> GLPVLNTPGSNQ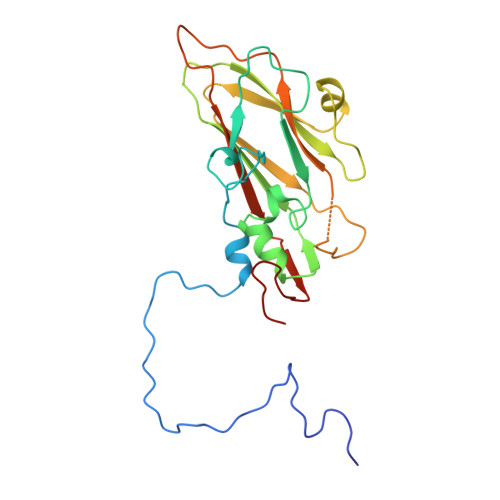YLTADNYQSPCAIPEFDVTPPIDIPGEVRNMMELAEIDTMIPLNLTNQRKNTMDMYRVELNDAAHSDTPILCLSLSPASDPRLAHTMLGEILNYYTHWAGSLKFTFLFCGSMMATGKLLVSYAPPGAEAPKSRKEAMLGTHVIWDIGLQSSCTMVVPWISNTTYRQTINDSFTEGGYISMFYQTRVVVPLSTPRKMDILGFVSACNDFSVRLLRDTTHISQEAMPQ4,5-dichlorobenzene-1,2-diol 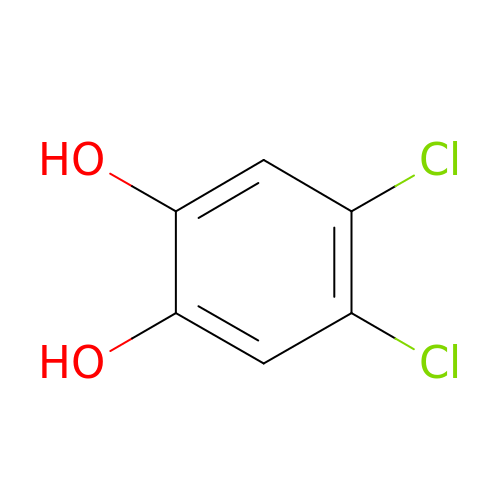| C6 H4 Cl2 O2 | ACCHWUWBKYGKNM-UHFFFAOYSA-N>[3x]MDTILLTGLFAAFFTTFAFAPQSIKTIRTRNTEGISVVMYIMFLTGVISWIAYGIMR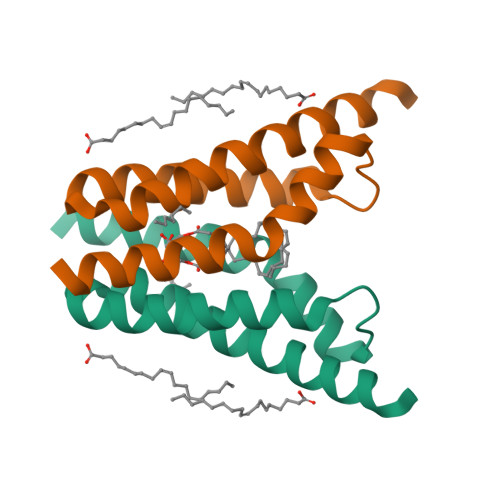SDFAVLIANIVTLFLAAPVLVITLINRRKKHVLESSGENLYFQ>[2x]HHHHHHFNL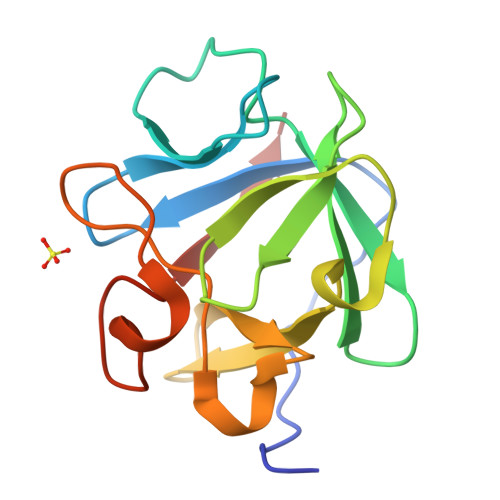PPGNYKKPKLLYCSNGGHFLRILPDGTVDGTRDRSDQHIQLQLSAESVGEVYIKSTETGQYLAMDTDGLLYGSQTPNEESLFLERLEENHYNTYISKKHAEKNWFVGLKKNGSCKRGPRTHYGQKAILFLPLPVSSD> PLGSRKCEKAGCTATCPVCFASASERCAKNGYTSRWYHLSCGEHFCNECFDHYYRSHKDGYDKYTTWKKIWTSNGKTEPSPKAFMADQQLPYWVQCTKPECRKWRQLTKEIQLTPQIAKTYRCGMKPNTAIKPETSDHCSLPEDLRVLEVSNHWWYSMLILPPLLKDSVAAPLLSAYYPDCVGMSPSCTSTNRAAATGNASPGKLEHSKAALSVHVPGMNRYFQPFYQPNECGKALCVRPDVMELDELYEFPEYSRDPTMYLALRNLILALWYTNCKEALTPQKCIPHIIVRGLVRIRCVQEVERILYFMTRKGLINTGVLSVGADQYLLPKDYHNKSVIIIGAGPAGLAAARQLHNFGIKVTVLEAKDRIGGRVWDDKSFKGVTVGRGAQIVNGCINNPVALMCEQLGISMHKFGERCDLIQEGGRITDPTIDKRMDFHFNALLDVVSE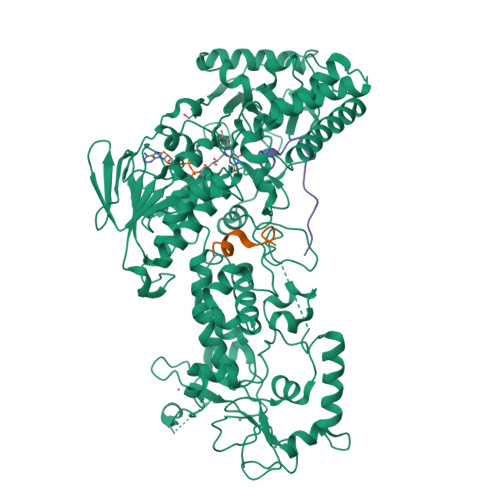WRKDKTQLQDVPLGEKIEEIYKAFIKESGIQFSELEGQVLQFHLSNLEYACGSNLHQVSARSWDHNEFFAQFAGDHTLLTPGYSVIIEKLAEGLDIQLKSPVQCIDYSGDEVQVTTTDGTGYSAQKVLVTVPLALLQKGAIQFNPPLSEKKMKAINSLGAGIIEKIALQFPYRFWDSKVQGADFFGHVPPSASKRGLFAVFYDMDPQKKHSVLMSVIAGEAVASVRTLDDKQVLQQCMATLRELFKEQEVPDPTKYFVTRWSTDPWIQMAYSFVKTGGSGEAYDIIAEDIQGTVFFAGEATNRHFPQTVTGAYLSGVREASKIAAF;> PLGSPEFSERGSKSPLKRAQEQSPRKRGRPPKDEKDLTIPESSTVKGMMAGPMAAFKWQPTASEPVKDADPHFHHFLLSQTEKPAVCYQAITKKLKICEEETGSTSIQAADSTAVNGSITPTDK;> ARTMQTARKSTGGKAPRKQLA> MHHHHHHSGMSLRLERDGAVARLLIDRADRRNAFSLDMWQRLPELLAEASGDDALRVLVVKSANGGA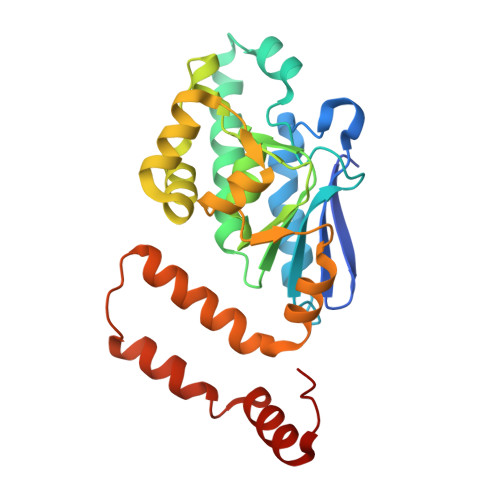FCAGADIAELLANKDDAAFHLANQQAINRAQYELARFRLPTVAMVEGDCIGGGCGIALACDMRIAAPAARFGITPAKLGLVYPLHDVKLLVDLVGPGQARRLMFTGGLIDANEAHRIGLVELLGESEDALVGQLATVSSFSTQAIKSFVRRVLDGQVADDTLSLCVFASATLGADFREGTGAFLEKRPPVF> MEYQLQQLASLTLVGIKETYENGRQAQQHIAGFWQRCYQEGVIADLQLKNNGDLAGILGLCIPELDGKMSYMIAVTGDNSADIAKYDVITLASSKYMVFEAQGAVPKAVQQKMEEVHHYIHQYQANTVKSAPFFELYQDGDTTSEKYITE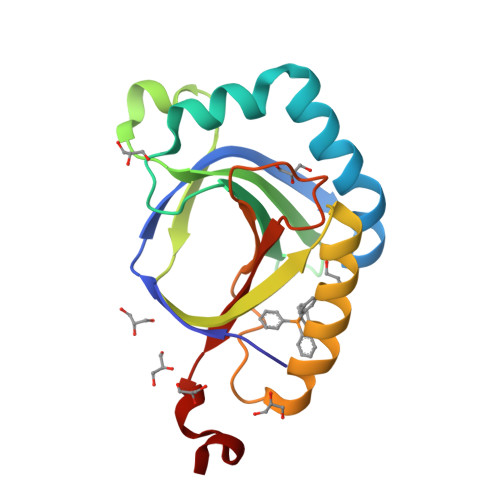IWMPVKGLEHHHHHH PNNs are a condensed form of neural extracellular matrix that include the glycosaminoglycan hyaluronan and extracellular matrix proteins such as aggrecan and tenascin-R (TNR). TNC and TNR share a common domain organization that includes an N-terminal cysteine-rich region responsible for the formation of disulfide-linked multimers, followed by 5-14 epidermal growth factor (EGF)-like domains, 8 to 9 FN repeats, and a C-terminal fibrinogen (Fg)-like domain. Here, we demonstrate that TNR and TNC associate with the single fibronectin type III (FN) domain found in RPTPζ and provide a structural basis of these interactions. Overall, our findings provide novel structural insights in the interactions between RPTPζ and tenascin family members, prove that the formation of a RPTPζ–TNR complex is essential to the assembly of PNNs, and provide a blueprint to explore a potential role for a RPTPζ–TNC complex in neural function.

Using sequence alignments, we identified two amino acid substitutions that could account for the lack of interaction between RPTPζ and TNN or TNX. First, Y2140 in TNC (Y1294 in TNR), whose side chain hydroxyl group makes a hydrogen bond to the main chain carbonyl group of Q369 in RPTPζ, is conserved in TNX but replaced by a histidine in TNN. Second, S2164 in TNC (S1318 in TNR) is conserved in TNN but replaced by a histidine in TNX. The effect of the Y2140H and S2164H mutations in the interactions between TNC and RPTPζ were thus analyzed in an Alpha-based competition binding assay. Introducing changes to histidine at positions Y2140 or S2164 prevented competition, suggesting that each mutation is enough to eliminate interaction with RPTPζ. Not surprisingly, a variant of TNC that includes both the Y2140H and S2164H mutations could not inhibit binding between RPTPζ and WT TNC. Finally, the crystal structure of this variant is identical to that of WT TNC, indicating that mutations at positions Y2140 or S2164 did not introduce any gross structural alteration that would account for the lack of interaction. Overall, these results validate our structural analyses of the interactions between RPTPζ, TNR, and TNC and explain why RPTPζ does not associate with additional tenascin family members.

>[2x]GTGSGLLYPFPKDCSQAMLNGDTTSGLYTIYLNGDKAEALEVFCDMTSDGGGWIVFLRRKNGRENFYQNWKAYAAGFGDRREEFWLGLDNLNKITAQGQYELRVDLRDHGETAFAVYDKFSVGDAKTRYKLKVEGYSGTAGDSMAYHNGRSFSTFDKDTDSAITNCALSHKGAFWYRNCHRVNLMGRYGDNNHHQGVNWFHWKGHEHSIQFAEMKLRPSNFRNLEGRRKRA>[4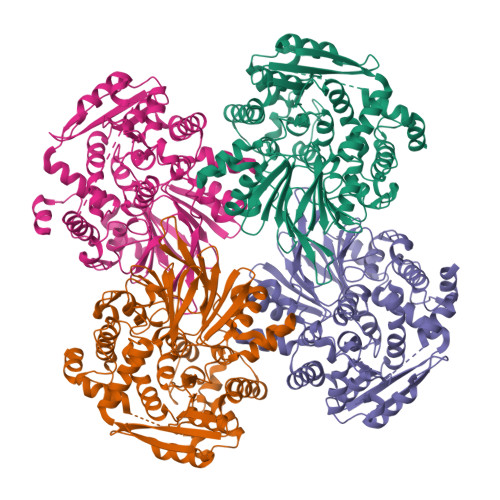x]MSNSFCVVYKGSDTDINNIQRDFDGKGEALSNGYLFIEQNGHYQKCEMERGTAYLIGSLYNRTFLIGLAGVWEGEAYLANDAELLALLFTRLGANALALAEGDFCFFIDEPNGELTVITESRGFSPVHVVQGKKAWMTNSLKLVTAAEGEGALWFEEEALVCQSLMRADTYTPVKNAQRLKPGAVHVLTHDSEGYSFVESRTLTTPASNQLLALPREPLLALIDRYLNAPLEDLAPRFDTVGIPLSGGLDSSLVTALASRHFKKLNTYSIGTELSNEFEFSQQVADALGTHHQMKILSETEVINGIIESIYYNEIFDGLSAEIQSGLFNVYRQAQGQVSCMLTGYGSDLLFGGILKPGAQYDNPNQLLAEQVYRTRWTGEFATHGASCYGIDIRHPFWSHSLISLCHALHPDYKIFDNEVKNILREYADSLQLLPKDIVWRKKIGIHEGSSVNQAFANVLGSTVDNYQTKSRFTYRVYQAFLRGRLSITDVTPSQLKDLIKKD>GVFTFEDE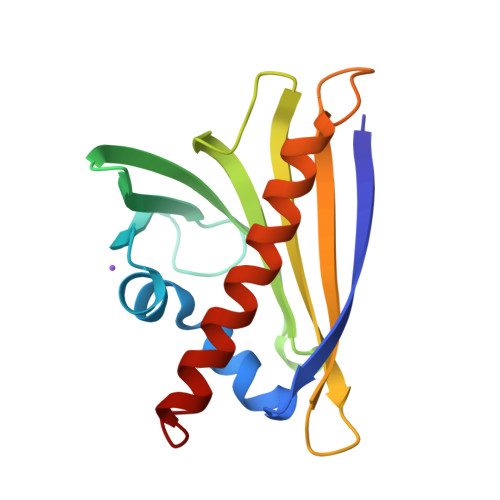ITSTVPPAKLYNAMKDADSITPKIIDDVKSVEIVEGNGGPGTIKKLTIVEDGETKFILHKVESIDEANYAYNYSVVGGVALPPTAEKITFETKLVEGPNGGSIGKLTLKYHTKGDAKPDEEELKKGKAKGEGLFRAIEGYVLANPTQY[2x]>[2x]MQKIGIYPGTFDPVTNGHIDIIHRSSELF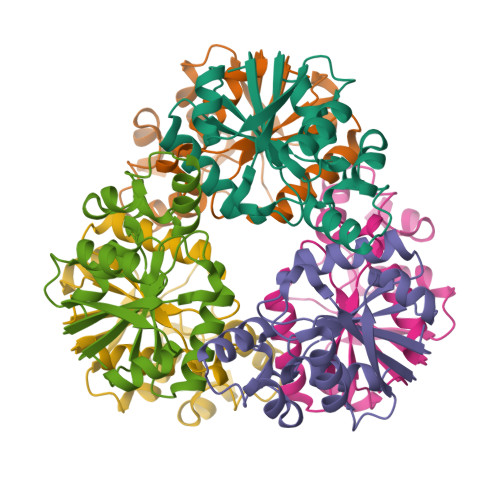EKLIVAVAHSSAKNPMFSLDERLKMIQLATKSFKNVECVAFEGLLANLAKEYHCKVLVRGLRVVSDFEYELQMGYANKSLNHELETLYFMPTLQNAFISSSIVRSIIAHKGDASHLVPKEIYPLISKA> RNDYVQEEKQQQLQEPLDGQWKPTTTGHDAIVPFSEPKPVTISEKAGVKFKPLLDVNTGCAPYAAVNAEGETSGGLQTSGDPESGCRGSKYGSQVYGRSTWYNDVWAIMYAWYFPKDSPMLLMGHRHDWENVVVFINDPDEVEPTILGCSTSWHSGYIKYAPCPTDSINGSSVMIKYEHSFPLNHALNITKDAGAYQDLIMWHQMPDLARRALNDTDFGKAITPMNDLNFMEKIEAAWPFKTKKDGA

Necrosis and ethylene inducing peptide 1 (Nep1)-like proteins (NLPs) are widely distributed among prokaryotic and eukaryotic organisms, like fungi, bacteria and oomycetes, and may infect a range of different crops, such as potato, tomato, soybean and tobacco, thus posing major threat to agriculture worldwide. It was shown that NLPs function as cytolytic toxins that induce plasma membrane leakage by binding to plant membrane sphingolipid receptor. NLPs share a conserved necrosis inducing protein (NPP1) domain, typically containing the heptapeptide motif, GHRHDWE, which is crucial for toxicity. The aim of the current study was to provide structural and functional information on similarities and differences between non-toxic HaNLP3 and toxic NLPPya, both members of the oomycete type 1 NLP group.

To investigate structural differences between non-toxic HaNLP3 and toxic NLPs, the HaNLP3 crystal structure was determined. The HaNLP3 structure comprises a nine-stranded β-sandwich flanked by three α-helices. The structure of HaNLP3 is defined in electron density from residue His28 to residue Thr242, and is thus missing 27 N-terminal and 5 C-terminal residues. Three glycosylated sites were observed at Asn169, Asn188 and Asn214. In addition, two bound phosphate ions were observed, likely due to the crystallization conditions. All amino acid residues involved in Mg2+ binding in NLPPya are preserved in HaNLP3 except for Asp158, which is also important for glucosamine binding in NLPPya and is replaced by Asn184 in HaNLP3. However, no metal ion is present in the HaNLP3 crevice. HaNLP3 Asn184 is involved in phosphate positioning, which is however mainly contributed to by the side chains of His125 and His154. Comparison of NLPPya protein surfaces in the apo- and hexose-bound states with HaNLP3 reveals that the crevice of HaNLP3 appears to be in a more closed state than the cavity of apo-NLPPya. Furthermore, HaNLP3 contains a second disulfide bond unlike NLPPya, which could play a part in HaNLP3 rigidity when interacting with the membrane.> GSSRGIPPKIEALPSDISIDEGKVLTVACAFTGEPTPEVTWSCGGRKIHSQEQGRFHIENTDDLTTLIIMDVQKQDGGLYTLSLGNEFGS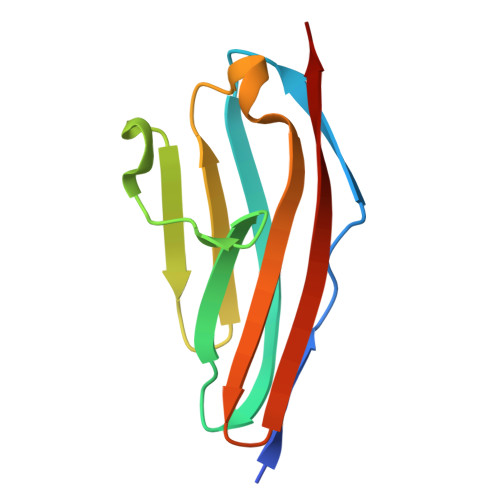DSATVNIHIRSI> YQ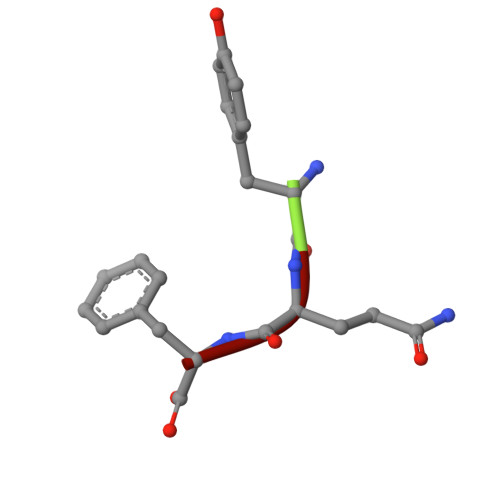F>[3x]MSQEIRQNEKISYRIEGPFFIIHLINPDNLNALEG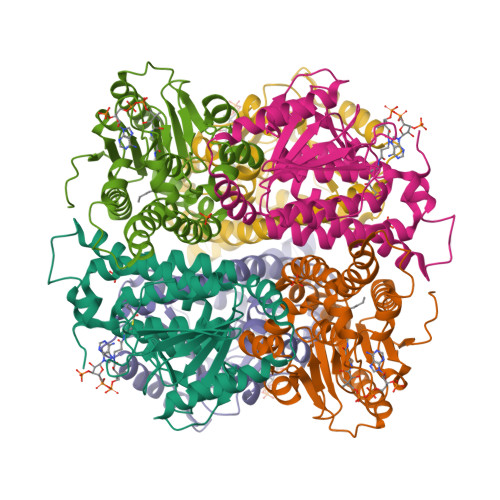EDYIYLGELLELADRNRDVYFTIIQSSGRFFSSGADFKGIAKAQGDDTNKYPSETSKWVSNFVARNVYVTDAFIKHSKVLICCLNGPAIGLSAALVALCDIVYSINDKVYLLYPFANLGLITEGGTTVSLPLKFGTNTTYECLMFNKPFKYDIMCENGFISKNFNMPSSNAEAFNAKVLEELREKVKGLYLPSCLGMKKLLKSNHIDAFNKANSVEVNESLKYWVDGEPLKRFRQLGSKQRKHRL> MQRKGTDEIYGLGSLPSAGPGRWEYLANPGNWHPERRKLHEKLLDQARSSALTLAESLESDGCQPTLFALRGNTATGKTRIATKKIPVLAAALKKTAGKGCVNPDVFKSSLAKSETGAKIFSSAQVHSESSFLADRFEGGLRSQKTGSGAIASIVVDKRLSREYEIDSYIQLAKETGRKVELCDIDAPLENSLVGVLQRKPEGEDPRPPYPVVSSGFVAVRSNRMYVIDRFIADPSLGNYRLFGTAEDGEKVMVASVIGGEFSVENAELYEKITSPQLSVTGDLADKVIDKELIDRLENNIAD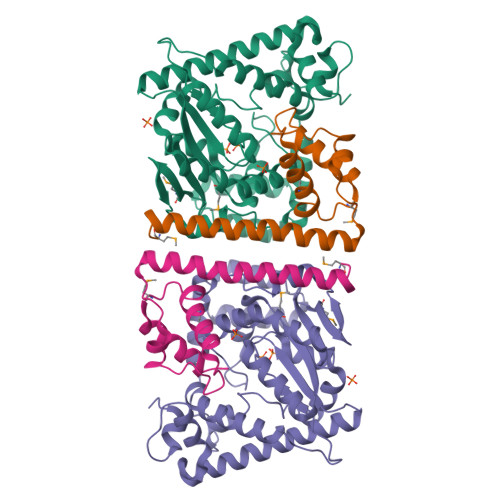PERAAKTRAALEKYSGKSWSAALAAHSELI;> MKTLTGADALEFHKKLKERNKALHASDLELALVHADAVGKERFDLEELEKICDTSDAGRLTDAKERNDIYERMYYVEYPNVMTLKEFAHIVETLFSWS>[2x]SNAMADRSVRPLRHLVHAVTGGQPPSEAQVRQAAWIARCVGRGGSAPLHRDDVSALAETLQVKEFAPGAVVFHADQTADGVWIVRHGLI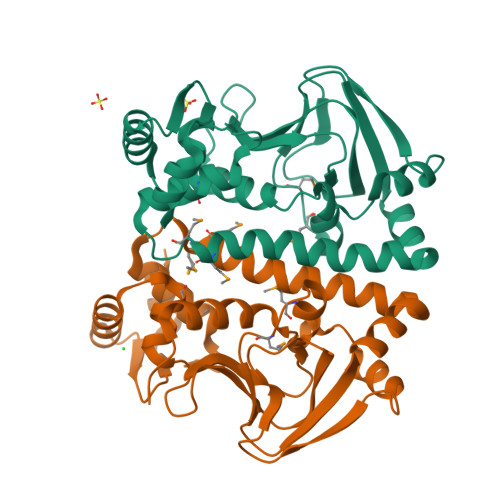ELAVGSRRRRAVVNILHPGDVDGDIPLLLEMPMVYTGRALTQATCLFLDRQAFERLLATHPAIARRWLSSVAQRVSTAQIRLMGMLGRPLPAQVAQLLLDEAIDARIELAQRTLAAMLGAQRPSINKILKEFERDRLITVGYAVIEITDQHGLRARAQ>MRGHHHHHHHGSMTIEFVGVEKIYPGGARSVRGVSFQIREGEMVGLLGPSGSGKTTILRLIAGLERPTKGDVWIGGKRVTDLPPQKRNVGLVFQNYALFQHMTVYDNVSFGLREKRVPKDEMDARVRELLRFMRLESYANRFPHELSGGQQQRVALARALAPRPQVLLFDEPFAAIDTQIRRELRTFVRQVHDEMGVTSVFVTHDQEEALEVADRVLVLHEGNVEQFGTPEEVYEKPGTLFVASFIGESNVWTRAVQNGRIEVAGAALPVDPAVSEGSEVAVVVRPKDVELQPASEREAHAQVVRSAFKGSYSACWIRTKDGEVWEVHVPSAD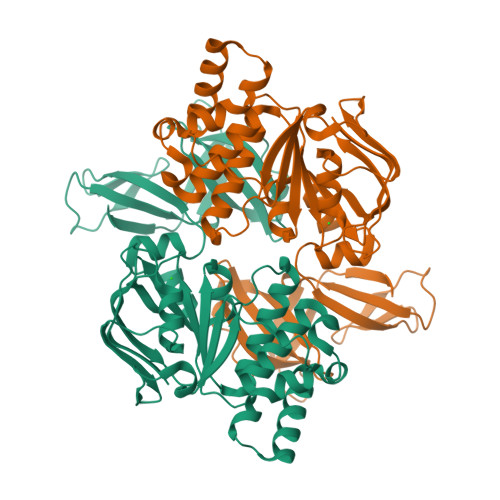RHRWSPGAWVHMNVTRWFIFPR[2x]> MKFKLNLITLALLANTGLAVAADGGSDGNNGNDGSDGGEPAGSIQTLNLDITKVSYENGAPMVTVFATNEADMPVIGLANLEIKKALQLIPEGATGPGNSANWQGLGSSKSYVDNKNGSYTFKFDAFDSNKVFNAQLTQRFNVVSAAGKLADGTTVPVAEMVEDFDGQGNAPQYTKNIVSHEVCASCHVEGEKIYHQATEVETCISCHTQEFADGRGKPHVAFSHLIHNVHNANKAWGKDNKIPTVAQNIVQDNCQVCHVESDMLTEAKNWSRIPTMEVCSSCHVDIDFAKGKGHSQQLDNSNCIACHNSDWTAELHTAKTTATKNLINQYGIETTSTINTETKAATISVQVVDANGTAVDLKTILPKVQRLEIITNVGPNNATLGYSGKDSIFAIKNGALDPKATINDAGKLVYTTTKDLKLGQNGADSDTAFSFVGWSMCSSEGKFVDCADPAFDGVDVTKYTGMKADLAFATLSGKAPSTRHVDSVNMTACANCHTAEFEIHKGKQHAGFVMTEQLSHTQDANGKAIVGLDACVTCHTPDGTYSFANRGALELKLHKKHVEDAYGLIGGNCASCHSDFNLESFKKKGALNTAAAADKTGLYSTPITATCTTCHTVGSQYMVHTKETLESFGAVVDGTKDDATSAAQSETCFYCHTPTVADHTKVKMSAWSHPQFEK

Bacterial multiheme cytochromes (MHCs) attract much attention for their contributions to extracellular electron transfer whereby electrons are exchanged across the cell boundary and consequently between internal enzymes and external redox partners. These processes evolved to allow the capture of electrons for anabolic reactions and the release of electrons from internal oxidation during anaerobic respiration. Thus, we investigated whether amber suppression in MR-1 could produce ncAA-containing MHCs and, specifically, variants of the MtrC protein, which contains ten c-type hemes. MtrC is found on the outer surface of MR-1 cells. MR-1 cells typically present MtrC tightly bound to the external face of the outer membrane spanning the MtrAB porin-cytochrome complex.

The structure of wtMtrC was inspected to identify surface residues that might be changed to ncAAs with limited effect on the MtrC structure. Residue A293 in Domain II and E344 and A430 in Domain III were chosen, Figure 2C. Thus, site-specific replacement of MtrC surface residues with BocK has no discernible impact on the protein structure. The current–potential profiles of the peaks for reduction (negative current) and oxidation (positive current) for all three BocK-containing proteins were highly similar to those of wtMtrC. For this reason, studies with the MtrC293BocK protein and the deletion strain were beyond the scope of this study.>[2x]SMRIGANGDETVWADEEFAGRDFRDEDLSRIRTERVVFTECDFSGVDLSESEHHGSAFRNCTFRRSTIWHSTFTNCSLLGSVFTECRIRPVTFVECDFTLAVLGGCDLRAVDLSDCRLREVSLVGADLRKAVLRRADLTGSRVQDARLEEADLRGTRVDPTFWTTAKVRGAK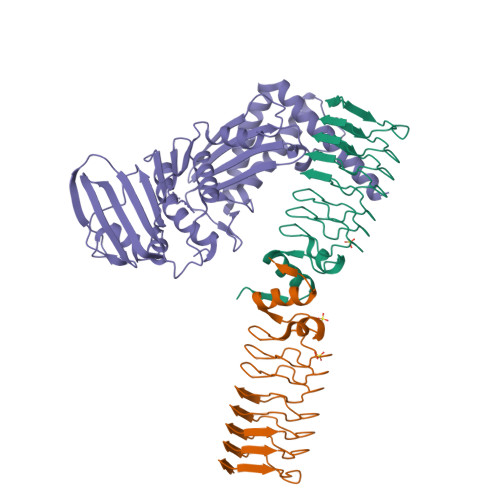IDIEQALAYAAAHGLAVHGG;> SMAAQKNNAPKEYGADSITILEGLEAVRKRPGMYIGSTGERGLHHLIWEVVDNAVDEAMAGFATRVDVKIHADGSVEVRDDGRGIPVEMHATGMPTIDVVMTQLHAGGKFDGETYAVSGGLHGVGVSVVNALSTRLEATVLRDGYEWFQYYDRSVPGKLKQGGETKETGTTIRFWADPEIFETTDYNFETVARRLQEMAFLNKGLTIELTDERVTAEEVVDDVVKDTAEAPKTADEKAAEATGPSKVKHRVFHYPGGLVDYVKHINRTKTPIQQSIIDFDGKGPGHEVEIAMQWNAGYSESVHTFANTINTHEGGTHEEGFRAALTSVVNRYAKDKKLLKDKDPNLTGDDIREGLAAVISVKVAEPQFEGQTKTKLGNTEVKSFVQKICNEQLQHWFEANPAEAKTVVNKAVSSAQARIAARKARELV>[2x]MSVHIEAKQGEIAESILLPGDPLRAKYIAETFLEDVTCYNNVRGMLGFTGTYKGKRVSVQG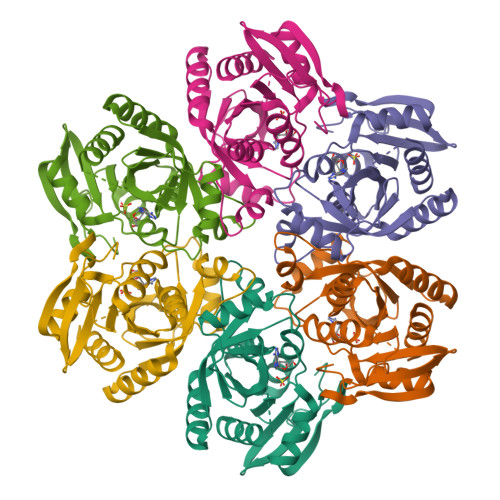TGMGVPSISIYVNELIQSYGVKNLIRVGTCGAIQKDVKVRDVIIAMTACTDSNMNRLTFPGFDFAPAANFDLLKKAYDAGTEKGLHVRVGNVLTADVFYRESMDMVKKLGDYGVLAVEMETTALYTLAAKYGVNALSVLTVSDHIFTGEETTSEERQTTFNEMIEIALDAAIQQ>[8x]MAATLLSPLSTHVLNIAQGVPGANMTIVLHRLDPVSSAWNILTTGITNDDG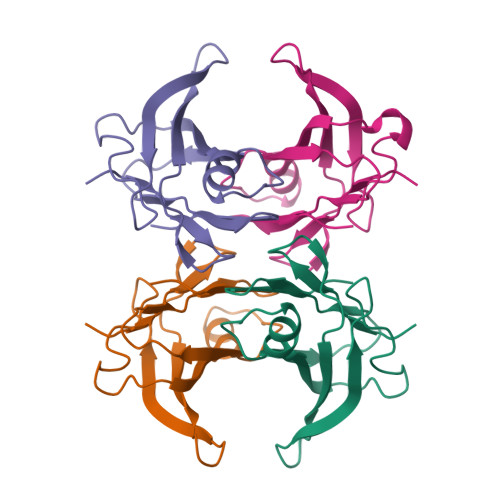RCPGLITKENFIAGVYKMRFETGKYWDALGETCFYPYVEIVFTITNTSQHYHVPLLLSRFSYSTYRGS> RLGEVEARQVATPREAQQLAQRQEAPKGEGL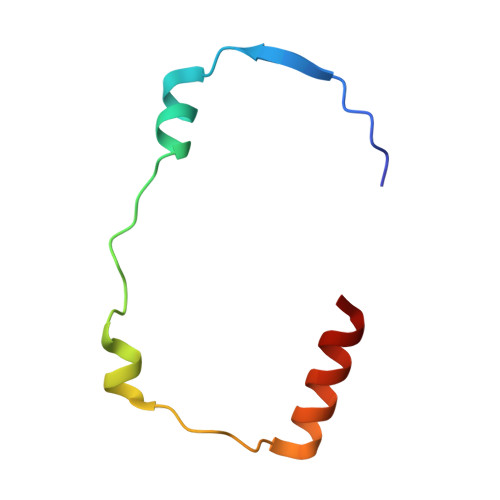LSRLGAALARPFVAIIEWLGKLLGSR>[2x]MSGAPPPSSGFAPRSYGQQPLSHAPRSSMMSVEYDGIPLPPPSIRSCGSQQYVTSYIPTGAAFPPSSVQDMISSMKSYASATDLVRTYSEIPSVEEALSTLDRAAAALNARRYRDALKLYLEGGYAMANVAERQANPKICNLLTSKGFETLNWCARLCDWIEGRIKEKHPRPGVHKVGIPVSNWDEDWVGPFMDEEEARRMWYTPVYCPHPIDFSNLGYRLRCVETGRRPRLMICITMYNEGPQQLKATLKKLANNLAYLKEQMPGDEKSLTGAFAGDDVWQNVLVCIVADGREQVHPKTLDYLEAIGLYDEDLLTINSAGIGAQCHLFEHTLQLSVNGKCLLPIQTVFALKENKASKLDSHHWYFNAFAEQIQPEYTAVMDVGTMLTKSALYHLLFAFERNHQIGGACGQLTVDNPFENLSNWVISAQHFEYKISNILDKSLESCFGFISVLPGAFSAYRYEAIRGAPLDAYFQTLNIELDVLGPFIGNMYLAEDRILSFEVVARKNCNWTMHYVKDAVARTDVPHDLVGLISQRKRWLNGAFFATLFSIWNWGRIYSESKHTFVRKMAFLVFYVYHLLYTAFGFFLPANLYLALFFIVFQGFQQNRLEFIDTSEYSQTVLDCAVYIYNFSYLFGLLMLIIIGLGNNPKHMKLTYYFVGAVFGLMMMLSSLVGAGIFFSTPATVHSIVVSILTVGVYFIASALHGEVHHIFMTFTHYTALIPSFVNIFTIYSFCNLQDLSWGTKGLHDDPLLAASLDETEKGDFKDVIAKRRALEELRREEKERVENRKKNFEAFRTNVLLTWAFSNLIFALFVVYFASSSTYMPVLYIFVASLNTCRLLGSIGHWVYIHTEGLRGRVIDKSECGNGTGRYPQNSYVQLEEHYAALAEDQRTYASGRTNASVRTVNDVSSAA

The core of the chitin biosynthetic machinery is an integral membrane enzyme named chitin synthase (CHS) (EC 2.4.1.16). Here we report five cryo-electron microscopy structures of a chitin synthase from the devastating soybean root rot pathogenic oomycete Phytophthora sojae (PsChs1). They represent the apo, GlcNAc-bound, nascent chitin oligomer-bound, UDP-bound (post-synthesis) and chitin synthase inhibitor nikkomycin Z-bound states of the enzyme, providing detailed views into the multiple steps of chitin biosynthesis and its competitive inhibition. The structures reveal the chitin synthesis reaction chamber that has the substrate-binding site, the catalytic centre and the entrance to the polymer-translocating channel that allows the product polymer to be discharged.

The apo structure of PsChs1 is the first example of a membrane-integrated processive glycosyltransferase with an apparently continuous but empty transmembrane channel, providing a real off-state of the enzyme before chitin synthesis is initiated. In the apo structure, it adopts a conformation different from those in the UDP-bound and UDP/(GlcNAc)3-bound states, with its carboxyl group pointing to the substrate-binding site, which may facilitate the recognition and correct positioning of the donor substrate at the substrate-binding site. Our PsChs1 structures revealed that the entrance to this channel is blocked by the swinging loop, specifically residue Pro454, in the apo and substrate-bound states, but it is open in the (GlcNAc)3-bound state. Molecular dynamics simulations of the apo and UDP/(GlcNAc)3-bound states of PsChs1 suggested that the VLPGA motif also acts as a permeability barrier that prevents water flux across the membrane in the apo state. PsChs1 was mainly purified as a dimer in solution. The two PsChs1 protomers are related to each other by a twofold rotation around an axis perpendicular to the membrane. Although TM topology algorithms predict IF3 to form a TM helix, our structures revealed that it actually forms a bent helix parallel to the membrane, as suggested previously for Chs3 in yeast. TM5 is an extraordinarily long helix (approximately 80 Å in length) that spans from the TM domain to the cytosolic region and projects into the opposite protomer like a sword. Two NTDs from the two PsChs1 protomers are wrapped by each other to form a symmetric and domain-swapped interface.> MALQSQASEEAKGPWQEADQEQQEPVGSPEPESEPEPEPEPEPVPVPPPEPQPEPQPLPDPAPLPELEFESERVHEPEPTPTVETRGTARGFQPPEGGFGWVVVFAATWCNGSIFGIHNSVGILYSMLLEEEKEKNRQVEFQAAWVGALAMGMIFFCSPIVSIFTDRLGCRITATAGAAVAFIGLHTSSFTSSLSLRYFTYGILFGCGCSFAFQPSLVILGHYFQRRLGLANGVVSAGSSIFSMSFPFLIRMLGDKIKLAQTFQVLSTFM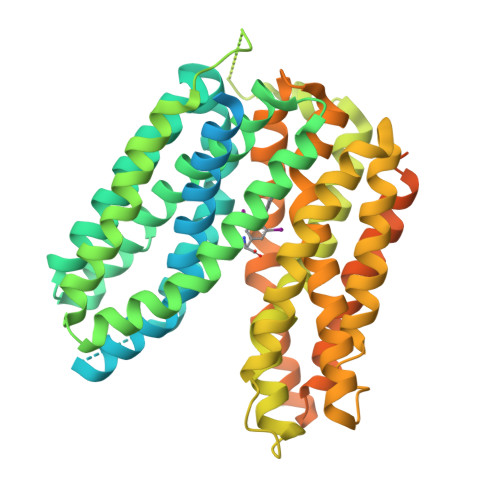FVLMLLSLTYRPLLPSSQDTPSKRGVRTLHQRFLAQLRKYFNMRVFRQRTYRIWAFGIAAAALGYFVPYVHLMKYVEEEFSEIKETWVLLVCIGATSGLGRLVSGHISDSIPGLKKIYLQVLSFLLLGLMSMMIPLCRDFGGLIVVCLFLGLCDGFFITIMAPIAFELVGPMQASQAIGYLLGMMALPMIAGPPIAGLLRNCFGDYHVAFYFAGVPPIIGAVILFFVPLMHQRMFKKEQRDSSKDKMLAPDPDPNGELLPGSPNPEEPIAAALEVLFQGPGAAEDQVDPRLIDGKHHHHHHHH Human Schlafen 11 (SLFN11) is sensitizing cells to DNA damaging agents by irreversibly blocking stalled replication forks, making it a potential predictive biomarker in chemotherapy. Furthermore, SLFN11 acts as a pattern recognition receptor for single-stranded DNA (ssDNA) and functions as an antiviral restriction factor, targeting translation in a codon-usage-dependent manner through its endoribonuclease activity. As a subgroup III Slfn family member, human SLFN11 has a tripartite domain architecture consisting of an N-terminal nuclease domain, followed by a linker domain and a C-terminal helicase domain. The N-terminal domains harbor its tRNA endoribonuclease active sites and the C-terminal helicase domains of the dimer are able to interact with ssDNA.

To understand the changes in the functional behavior of SLFN11S753D and to provide a structural basis for the regulatory role of the S753 phosphorylation, we employed cryo-EM to determine the structure of the phosphomimetic SLFN11 Ser 753 to Asp mutant bound to ATP. SLFN11S753D yielded exclusively monomeric 2D classes, which is in contrast to the predominantly dimeric state that was previously observed for SLFN11wt 26. To counteract preferred particle orientation, cryo-EM data of SLFN11S753D were recorded at a tilt angle of 25°. This resulted in a 3D reconstruction of monomeric SLFN11S753D with a global resolution of 3.72 Å, allowing model building of residues 7-897. The SLFN11S753D cryo-EM sample was prepared in the presence of ATP, which is in line with the observation of additional density in the nucleotide-binding pocket, suggesting a nucleotide bound state. ATP is coordinated by the Walker A and B motifs that are responsible for ATP binding and hydrolysis. The conserved glutamine residue of the Q-motif coordinates the adenine base. The same region adopts a vastly different conformation in SLFN11S753D, disrupting the long ID-helix, and forming a more open conformation. The conformational change of the ID-region between SLFN11wt and SLFN11S753D is accompanied by a rotation of the entire helicase domain by approximately 140°. The loss of dimer interface I, as a result of the rotated helicase domains, likely destabilizes the dimeric state, explaining why SLFN11S753D adopts a solely monomeric state in solution. In this conformation, SLFN11S753D is unable to bind ssDNA, but is proficient in ATP binding, though not in hydrolysis and has diminished tRNA cleavage activity.

> MADYKDDDDKGTDYKDDDDKLEVLFQGPMEANQCPLVVEPSYPDLVINVGEVTLGEENRKKLQKIQRDQEKERVMRAACALLNSGGGVIRMAKKVEHPVEMGLDLEQSLRELIQSSDLQAFFETKQQGRCFYIFVKSWSSGPFPEDRSVKPRLCSLSSSLYRRSETSVRSMDSREAFCFLKTKRKPKILEEGPFHKIHKGVYQELPNSDPADPNSDPADLIFQKDYLEYGEILPFPESQLVEFKQFSTKHFQEYVKRTIPEYVPAFANTGGGYLFIGVDDKSREVLGCAKENVDPDSLRRKIEQAIYKLPCVHFCQPQRPITFTLKIVNVLKRGELYGYACMIRVNPFCCAVFSEAPNSWIVEDKYVCSLTTEKWVGMMTDTDPDLLQLSEDFECQLSLSSGPPLSRPVYSKKGLEHKKELQQLLFSVPPGYLRYTPESLWRDLISEHRGLEELINKQMQPFFRGILIFSRSWAVDLNLQEKPGVICDALLIAQNSTPILYTILREQDAEGQDYCTRTAFTLKQKLVNMGGYTGKVCVRAKVLCLSPESSAEALEAAVSPMDYPASYSLAGTQHMEALLQSLVIVLLGFRSLLSDQLGCEVLNLLTAQQYEIFSRSLRKNRELFVHGLPGSGKTIMAMKIMEKIRNVFHCEAHRILYVCENQPLRNFISDRNICRAETRKTFLRENFEHIQHIVIDEAQNFRTEDGDWYGKAKSITRRAKGGPGILWIFLDYFQTSHLDCSGLPPLSDQYPREELTRIVRNADPIAKYLQKEMQVIRSNPDFNIPTGCLEVFPEAEWSQGVQGTLRIKKYLTVEQIMTCVADTCRRFFDRGYSPKDVAVLVSTAKEVEHYKYELLKAMRKKRVVQLSDACDMLGDHIVLDSVRRFSGLERSIVFGIHPRTADPAILPNVLICLASRAKQHLYIFPWGGH A plant called Arabidopsis thaliana has a light-sensitive protein called ZEITLUPE (or ZTL for short) that helps it keep its circadian clock in sync with the cycle of night and day. In Arabidopsis thaliana, three LOV domain containing proteins ZTL, FLAVIN-BINDING, KELCH REPEAT, F-BOX 1 (FKF1), and LOV KELCH PROTEIN 2 (LKP2) act in circadian timing and seasonal flowering. Recent research indicates that their divergent roles in the circadian clock and photoperiodic flowering may enable interrogation of how chemistry regulates PAS/LOV protein function to select for signaling pathways. These proteins retain analogous elements, where an N-terminal LOV domain regulates activity of a C-terminal E3 ubiquitin ligase to target clock proteins for degradation in a time dependent manner. LOV domains are typified by blue-light induced formation of a C4a adduct between a conserved Cys residue and a bound flavin (FAD, FMN or riboflavin) cofactor.

Towards these aims we solved 2.5 Å, 2.6 Å, and 2.1 Å crystal structures of dark-state WT ZTL, G80R and V48I:G80R (residues 29–165) respectively. Namely, G80R structures are analogous to WT in all manners. The primary difference is the formation of a π-cation interaction that stabilizes the Dα/Eα linkage and C82 that is necessary for C4a adduct formation. Increased rigidity of C82 imposed by the π-cation interaction is consistent with having an effect only on photocycle kinetics. R80 within Dα forms a π-cation interaction with F84 directly above the photoreactive C82, resulting in steric stabilization of adduct formation. The observed steric stabilization through the π-cation interaction is consistent with the longer photocycle in G80R. In ZTL, Q154 does not adopt a specific orientation as observed in all other LOV structures, rather it varies in all four molecules in the asymmetric unit of both WT-ZTL and G80R. G80R does not impact ZTL structure or allosteric regulation of Ncap or Ccap elements. In this manner, G80R acts as a photocycle variant only and allows direct testing of LOV photocycle kinetics on targeted degradation of PRR5 and TOC1 (see Equation 1). The G80R variant, likely due to the stabilizing effects of the R80-F84 π-cation interaction, enhances protein yields in E. coli substantially.

>[4x]GGPIPYPVGNLLHTAPCGFVVTDAVEPDQPIIYVNTVFEMVTGYRAEEVLGRNCRFLQCRGPFAKRRHPLVDSMVVSEIRKCIDEGIEFQGELLNFRKDGSPLMNRLRLTPIYGDDDTITHIIGIQFFIETDIDLGP> STMAIEKILTDAKTLLERLREHDAAAESLVDQSAALHRRVAAMREAGTALPDQYQEDASDMKDMS;> STMEQLSQYLQEALHREQM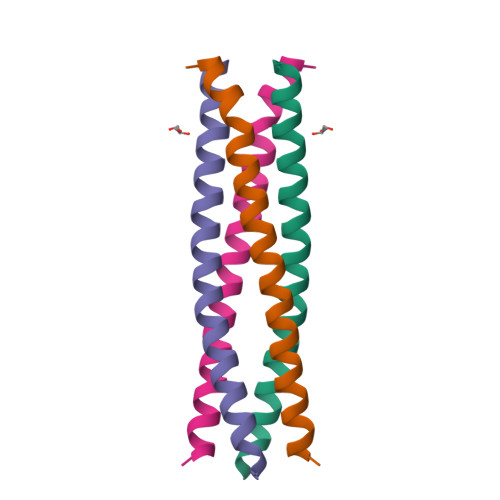LEQKLATLQRLLAITQEASDTSWQALIDEDRLLSRLEVMGNQLQA>[3x]MNQNLLVTKRDGSTERINLDKIHRVLDWAAEGLHNVSISQVELRSHIQFYDGIKTSDIHETIIKAAADLISRDAPDYQYLAARLAIFHLRKKAYGQFEPPALYDHVVKMVEMGKYDNHLLED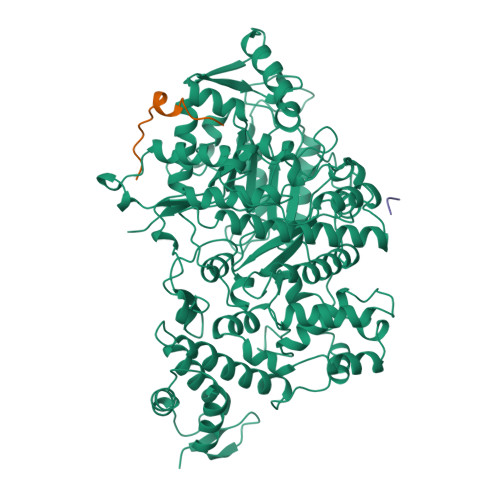YTEEEFKQMDTFIDHDRDMTFSYAAVKQLEGKYLVQNRVTGEIYESAQFLYILVAACLFSNYPRETRLQYVKRFYDAVSTFKISLPTPIMSGVRTPTRQFSSCVLIECGDSLDSINATSSAIVKYVSQRAGIGINAGRIRALGSPIRGGEAFHTGCIPFYKHFQTAVKSCSQGGVRGGAATLFYPMWHLEVESLLVLKNNRGVEGNRVRHMDYGVQINKLMYTRLLKGEDITLFSPSDVPGLYDAFFADQEEFERLYTKYEKDDSIRKQRVKAVELFSLMMQERASTGRIYIQNVDHCNTHSPFDPAIAPVRQSNLCLEIALPTKPLNDVNDENGEIALCTLSAFNLGAINNLDELEELAILAVRALDALLDYQDYPIPAAKRGAMGRRTLGIGVINFAYYLAKHGKRYSDGSANNLTHKTFEAIQYYLLKASNELAKEQGACPWFNETTYAKGILPIDTYKKDLDTIANEPLHYDWEALRESIKTHGLRNSTLSALMPSETSSQISNATNGIEPPRGYVSIKASKDGILRQVVPDYEHLHDAYELLWEMPGNDGYLQLVGIMQKFIDQSISANTNYDPSRFPSGKVPMQQLLKDLLTAYKFGVKTLFYQNTRDGAEDAQDDLVPSIQDDGCESGACKI;>YLVGQIDSEVDTDDLSNFQL[4x]> ADQPSPTWGIDRIDQRNLPLDNNYHTDYDGSGVTAFVIDTGVLNTHNEFGGRASSGYDFIDNDYDATDCNGHGTHVAGTIGGSTYGVAKNVNVVGVRVLNCSGSGSNSG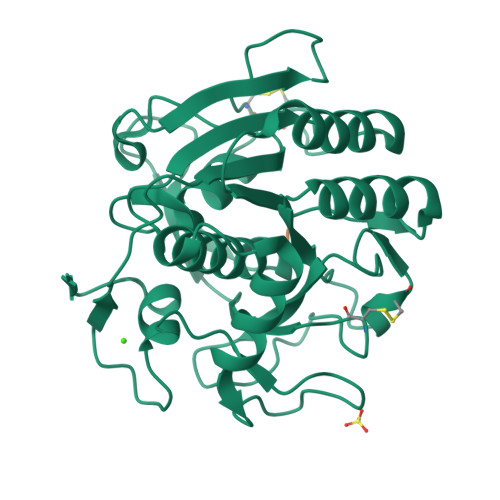VIAGINWVKNNASGPAVANMSLGGGASQATDDAVNAAVAAGITFVVAAGNDNSNACNYSPARAADAITVGSTTSNDSRSSFSNYGTCLDIYAPGSSITSSWYTSNSATNTISGTSMASPHVAGVAALYLDENPNLSPAQVTNLLKTRATADKVTDAKTGSPNKLLFSLA;> APT>GPMGTDWPVYHRIDGPIVMIGFGSIGRGTLPLIERHFAFDRSKLVVIDPSDEARKLAEARGVRFIQQAVTRDNYRELLVPLLTAGPGQGFCVNLSVDTSSLDIMELARENGALYIDTVVQPWLGFYFDPDLKPEARSNYALRETVLAARRNKPGGTTAVSCCGANPGMVSWFVKQALVNLAADLGVTGEEPTTREEWARLAMDLGVKGIHIAERDTQRASFPKPFDVFVNTWSVEGFVSEGLQPAELGWGTFERWMPDNA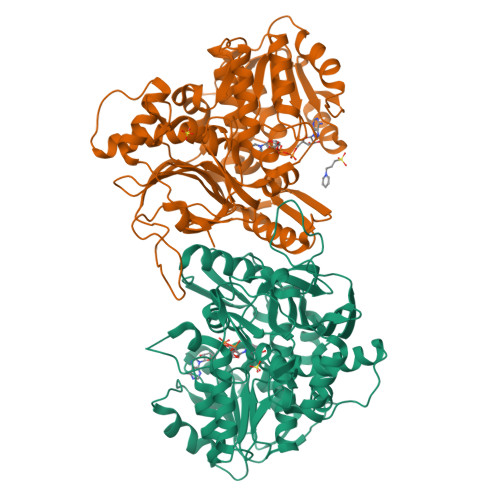RGHDSGCGAGIYLLQPGANTRVRSWTPTAMAQYGFLVTHNESISIADFLTVRDAAGQAVYRPTCHYAYHPCNDAVLSLHEMFGSGKRQSDWRILDETEIVDGIDELGVLLYGHGKNAYWYGSQLSIEETRRIAPDQNATGLQVSSAVLAGMVWALENPNAGIVEADDLDFRRCLEVQTPYLGPVVGVYTDWTPLAGRPGLFPEDIDTSDPWQFRNVLVRD[2x]>MPQDVDFHIPLPGRQSPDHARAEAEQLAWPRSLGLIRSDAAAERHLRGGYADLASRFYPHATGADLDLGVDLMSWHFLFDDLFDGPRGENPEDTKQLTD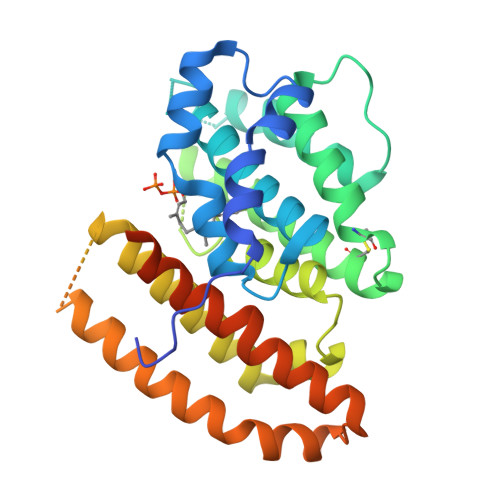QVAAALDGPLPDTAPPIAHGFADIWRRTCEGMTPAWCARSARHWRNYFDGYVDEAESRFWNAPCDSAAQYLAMRRHTIGVQPTVDLAERAGRFEVPHRVFDSAVMSAMLQIAVDVNLLLNDIASLEKEEARGEQNNMVMILRREHGWSKSRSVSHMQNEVRARLEQYLLLESCLPKVGEIYQLDTAEREALERYRTDAVRTVIRGSYDWHRSSGRYDAEFALAAGAQGYLEELGSSAH[2x]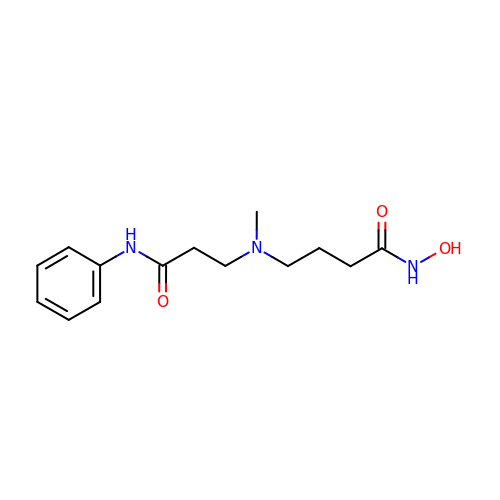4-[(3-anilino-3-oxopropyl)(methyl)amino]-N-hydroxybutanamide | C14 H21 N3 O3 | XWKAYUOSXSESEL-UHFFFAOYSA-N>GAMGRILFLTTFMSKGNKVVRYLESLHHEVVICQEKVHAQSANLQEIDWIVSYAYGYILDKEIVSRFRGRIINLHPSLLPWNKGRDPVFWSVWDETPKGVTIHLIDEHVDTGDILVQEEIAFADEDTLLDCYNKANQAIEELFIREWENIVHGRIAPYRQTAGGTLHFKADRDF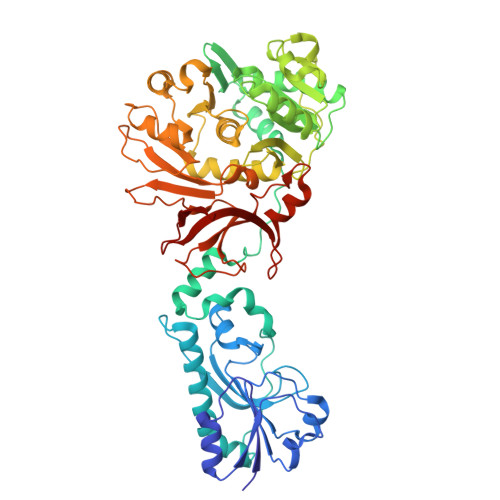YKNLNMTTVRELLALKRLCAEPKRGEKPIDKTFHQLFEQQVEMTPDHVAVVDRGQSLTYKQLNERANQLAHHLRGKGVKPDDQVAIMLDKSLDMIVSILAVMKAGGAYVPIDPDYPGERIAYMLADSSAAILLTNALHEEKANGACDIIDVHDPDSYSENTNNLPHVNRPDDLVYVMYTSGSTGLAKGVMIEHHNLVNFCEWYRPYFGVTPADKALVYSSFSFDGSALDIFTHLLAGAALHIVPSERKYDLDALNDYCNQEGITISYLPTGAAEQFMQMDNQSFRVVITGGDVLKKIERNGTYKLYNGYGPTECTIMVTMFEVDKPYANIPIGKPIDRTRILILDEALALQPIGVAGELFIVGEGLGRGYLNRPELTAEKFIVHPQTGERMYRTGDRARFLPDGNIEFLGRLD[4x]> MTTLLNPYFGEFGGMYVPQILMPALNQLEEAFVSAQKDPEFQAQFADLLKNYAGRPTALTKCQNITAGTRTTLYLKREDLLHGGAHKTNQVLGQALLAKRMGKSEIIAETGAGQHGVASALASALLGLKCRIYMGAKDVERQSPNVFRMRLMGAEVIPVHSGSATLTDACNEALRDWSGSYETAHYMLGTAAGPHPYPTIVREFQRMIGEETKAQILDKEGRLPDAVIACVGGGSNAIGMFADFINDTSVGLIGVEPGGHGIETGEHGAPLKHGRVGIYFGMKAPMMQTADGQIEESYSISAGLDFPSVGPQHAYLNSIGRADYVSITDDEALEAFKTLCRHEGIIPALESSHALAHALKMMREQ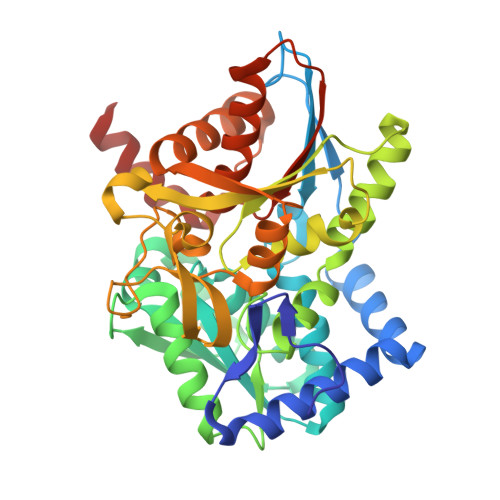PEKEQLLVVNLSGRGDKDIFTVHDILKARGEI>MIDVIMTGELLKTVTRAIVALVSEARIHFLEKGLHSRAVDPANVAMVIVDIPKDSFEVYNIDEEKTIGVDMDRIFDISKSISTKDLVELIVEDESTLKVKFGSVEYKVALIDPSAIRKEPRIPELELPAKIVMDAGEFKKAIAAADKISDQVIFRSDKEGFRIEAKGDVDSIVFHMTETELIEFNGGEARSMFSVDYLKEFCKVAGSGDLLTIHLGTNYPVRLVFELVGGRAKVEYILAPRIESE[3x];>GPLGSPEFPGRLMKAGIDEAGKGCVIGPLVVAGVACSDEDRLRKLGVKDSKKLSQGRREELAEEIRKICRTEVLKVSPENLDERMAAKTINEILKECYAEIILRLKPEIAYVDSPDVIPERLSRELEEITGLRVVAEHKADEKYPLVAAASIIAKVEREREIERLKEKFGDFGSGYASDPRTREVLKEW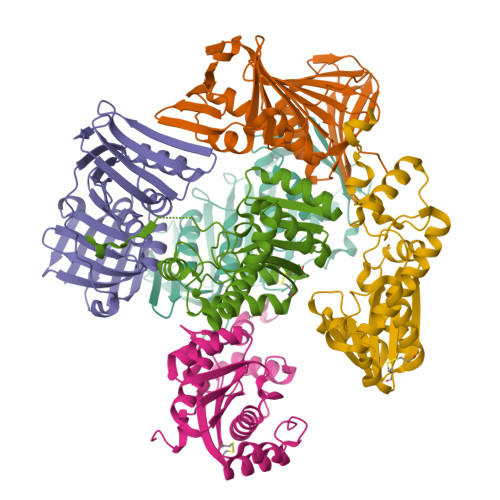IASGRIPSCVRMRWKTVSNLRQKTLDDF[3x]>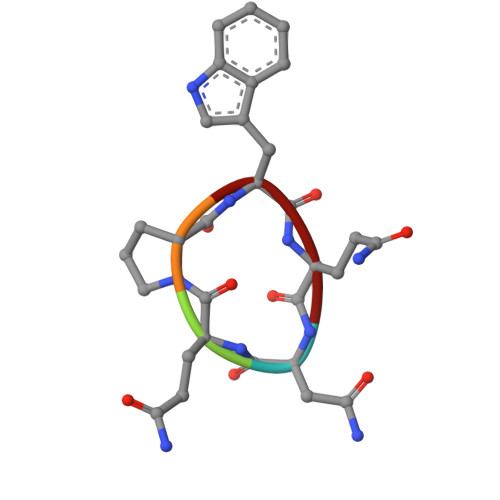 NQPWQ> ACEMCRLGLPHGSFFELLRDWKKIEE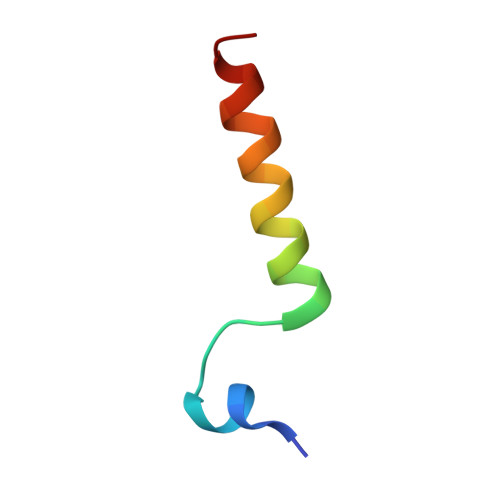FRNKS>[2x]MVLKITDIEVLHLRVPAMDADCEWGEDAVIVKVHTDKGIVGVGEADSSPLVVQACIEAPQTNFYCNGLKRLLIGENALEIERLWNKMYWGSNYMGRRGAGIHAISAIDIALWDIAGQFYGVPVHTLLGGKYRDKIRCYGTFIPADKPEDNVAIVQGLKDQGFSSIKFGGGVMGDDPDTDYAIVKAVREAAGPEMEVQIDLASKWHTCGHSAMMAK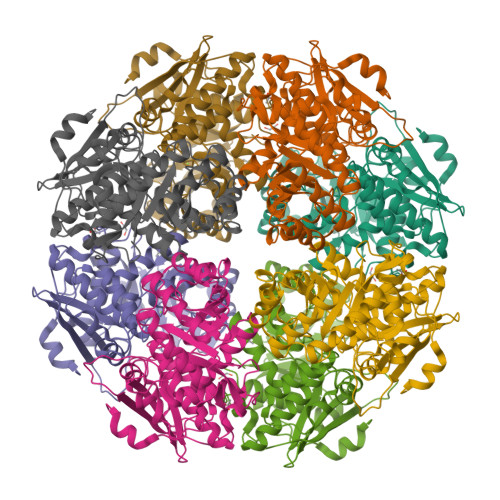RLEEFNLNWIEEPVLADSLISYEKLSRQVSQKIAGGESLTTRYEFQEFITKSNADIVQPDITRCGGITEMKKIYDIAQMNGTQLIPHGFSTGILLHASVHFLAACEQGTLMEFSQSSSPLFTSLVKNQLQFDNGFVAVSDAPGLGIELDEELIAKYRVN>GHPFVSIADSILDNVLNLYQTEDGLLTETYPVNPDQKITYLAGGAQQNGTLKASFLWPYSGMMSGCVAMYQATGDKKYKTILEKRILPGLEQYWDGERLPACYQSYPVKYGQHGRYYDDNIWIALDYCDYYRLTKKADYLKKAIALYEYIYSGWSDELGGGIFWCEQQKEAKHTCSNAPSTVLGVKLYRLTKDKKYLNKAKETYAWTRKHLCDPDDFLYWDNINLKGKVSKDKYAYNSGQMIQAGVLLYEETGDKDYLRDAQKTAAGTDAFFRSKADKKDPSVKVHKDMSWFNVILFRGFKALEKIDHNPTYVRAMAE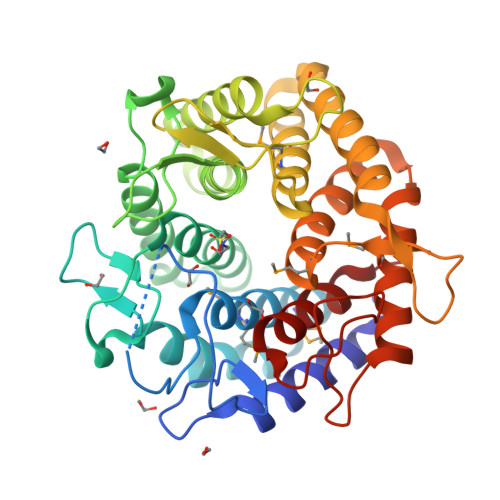NALHAWRNYRDANGLLGRDWSGHNEEPYKWLLDNACLIELFAEIEK[2x]>SHMFTSLEGRSAIVTGGSKGIGRGIAETFANAGVDVVITGRNQDDLDRTVADLSGTRGKVTAVRADVTDPEDARRTVAETVSRHGGLDIV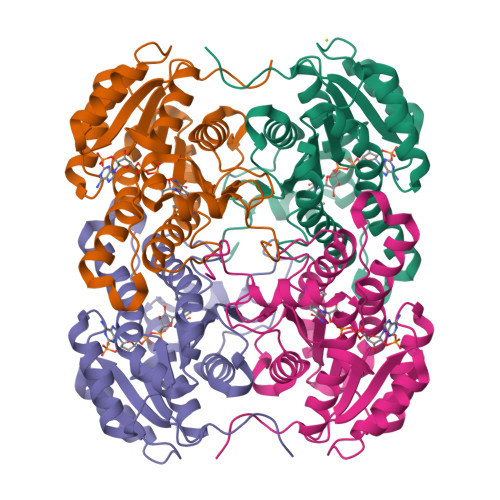CANAGIFPSGRLEDLTPDDIEQVLGVNFKGTVYIVQAALQALTASGHGRVVVTSSITGPITGYPGWSHYGASKAAQLGFLRTAAMELAPKKITINAVLPGNIMTEGLDEMGQDYLDQMASAIPAGRLGSVADIGNAALFFATDEAAYVTGQTLVVDGGQVLPESHLAIA[16x]>[2x]MGKVPETHKGYVFTSGSSRLTLKDVPTYKPGPGEVLLKLEASGVCHSDLHILQGSFPIPSNSVLGHEITGTVVAYGLGVDPKTYPEGQLYAAHGPNPCGSCRECRSGKDNLCHAENRTNYGLGYPGGYQQYTLAKVHNLIKVPDGVGAAIAAVTTDAVLTPYHAFKKADINGLSKILIIGLGGLGINAVQIAKAMGAHVTAYDLKESSRQ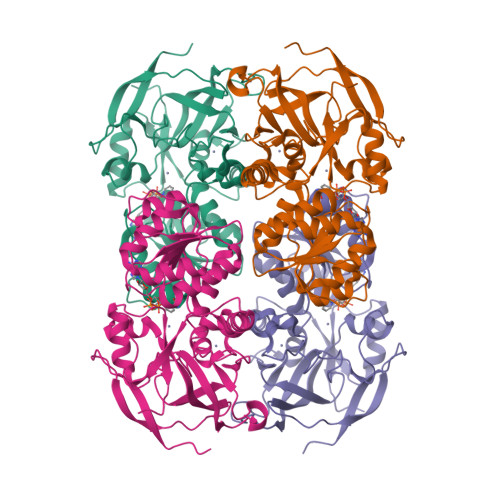LARQFGADVVLESLTLDDASKEYDFVADIVSIQSTFDLALKQVKSNGLVIPLGLGSPKLTFDQNDLLVREIRILGSFWGTSLDQAEVFDLVKSGAFKPQVETGKFKDLNEILEKLEKGQIKSRLVLTDFDDIMASMTGGQQMGRDPNSSSVDKLAAALEHHHHHH>GEDDYYYPSVKLEFVTVKAGTDGSIQTLIPDNGEALTVSKDRTGSAISPNTSRRVMSNYETLSNGHTATAVIYSLQSLVTPTPKPADDPTYRDGLKHDPVDVVSIWLGRGYLNMILNLKVNGGKQHVFGIVEDLSEFETNGTVNMLLYHDANGDEEYYNRRAYLSVPLDKYADAENPGQKITIKFKY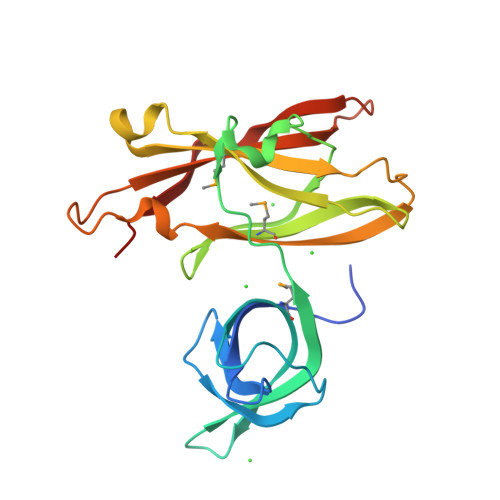YTYDKDGTAIESGKYCNPGFEYVPDKN[12x]> TPDSIDYRKKGYVTPVKNQGQCGSCWAFSSVGALEGQLKKKTGKLLNLSPQNLVDCVSENDGCGGGYMTNAFQYVQRNRGIDSEDAYPYVGQDESCMYNPTGKAAKCRGYREIPEGNEKALK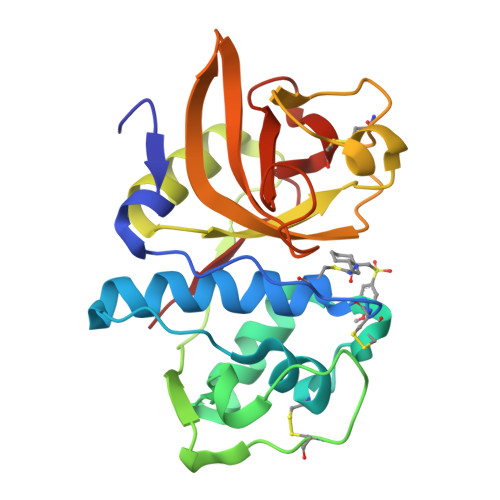RAVARVGPVSVAIDASLTSFQFYSKGVYYDENCSSDNLNHAVLAVGYGIQKGNKHWIIKNSWGESWGNKGYILMARNKNNACGIANLASFPKM> MYGTGTGPQTGAVTPRSSASLRPLTLSHGSLETSFLIPTGLHFHASRLKDEFIASLPPPTDELAQDDEPSSVPELVARYMGYIANQVAEGEDDAQGSYEEVLKLILNEFERAFLQGNDVHALVATLPGIDAKKLEVIRSYFAARAATNRAMRAHQSALLRAAEEGEARIYSIFGGQGNIEEYFEELRELYKTYPSFVGHLIVSSAELLQILASHPSAEKLYSKGLDIMHWLHNPDATPDTDYLISAPVSFPLIGLVQLAHYQVTCKVQGLHPGILRDRISGTTGHSQGIVLAAVTAAADSWESFEDLAKSALTILFWIGARSQQTFPRTSMSPSLLQEAIDNGEGTPTPMLSIRDLPQAEVQKHIDQTNQYLPEDQHISISLINSPRNLVVSGPPRSLCGLNAQLRKVKAPTGLDQARIPYSERKIRFVNRFLPITAPFHSKYLAGAAELIAEDLKDISIEVERLGIPVYDTNTGEDIRQTVTGNVVPALIRMITNDPVHWEKATVFPEATHILDFGPGGISGLGVLTSRNKDGTGVRVILAGTVNGTVAEVGYKSELFDRDEEHAVKYAVDWVKEYGPRLIKTSSGRIYVDTKMSRLLGLPPLMVAGMTPTTVPWDFVAATMNAGYQIELAGGGYFNAKMMTEAISKIERAIPPGRGITVNLIYVNPHAMAWQIPLLGRLRAEGVPIEGLTIGAGVPSIEVANEYIQTLGLKHISFKPGSVDAIQAVINIAKANPTFPVILQWTGGRGGGHHSYEDFHAPILAMYSRIRRQENIILVAGSGFGGAEDTYPYLTGAWSTKYGYPPMPFDGCLFGSRMMVAKEAHTSPEAKQAIVDAPGLDDSEWEKTYKGPAGGVITVRSEMGEPIHKLATRGVLFWAEMDQKIFSLPKEKRVAELKKNRDYIIRKLNADFQKVWFGKNKKGEVVDLEDMTYGEVVRRMVELLYVKDEKRWIDHSFAKLTADFIHRVEERFTTAASQPSLIQSYSDLDEPYSAVERVLAHYPEAETQLISAQDVQHFLLLCKRRGQKPVTFVPALDEDFEFYFKKDSLWQSEDLAAVIDRDVGRTCILQGPMAAKHSTKVDEPIKEILDGIHNGHIAALKRDLYDNDESKIPTIEYFGGKLKDPEVQLDFEGVTISYDVHKNTYRVSNNPSVPLPPLDAWLSALAGPNRTWRYALLQSEVIVQGHKYQTNPMKKIFAPARGLFVEIQYPNDPAKTVITVKEQPRPNRYIDVIEAKLVGDKEIVVNLIKDTNALGEPVALPLRFTYRPEAGYAPIHEIMEGRNDRIKEFYWRCWFGQDPLDLDAPVTSKFDGGEAVITSEAINEFVHAVGNTGEAFVDRPGKTMYAPMDFAIVVGWKAITKPIFPRTIDGDLLKLVHLSNQFRMFPGAEPLKKGDKVYTTAQVNAVINQESGKMVEVCGTITRDGKPVMEVISQFLYRGVYTDYENTFQRKVETPMQVHLATTKDIAILRSKQWFVLDDVATPEEFLLGKTLTFRLHTLVHFKNRNVYSHVETRGQVLVELPTKEIIQVATVEYVAGESHGNPVIDYLQRNGQSIEQPVNFENPIPLGGKAPLQLRAPASNETYARVSGDYNPIHVSRVFAAYANLPGTITHGMYSSAAVRSLVETWAAENKIGRVRSFHASLTGMVLPNDDINVKLQHVGMVGGRKIIKVEATNKETEEKVLLGEAEIEQPVTAYVFTGQGSQEQGMGMDLYANSPVAREVWDRADKYLRDTYGFAITDIVRNNPKELTIHFGGPLGKKIRANYMAMTFETVAADGSIKSERIFKDIDENTTSYTFRSPNGLLSATQFTQPALTLMEKASFEDMKAKGLVPRDSTFAGHSLGEYSALAALADVMPIESLVSVVFYRGLTMQV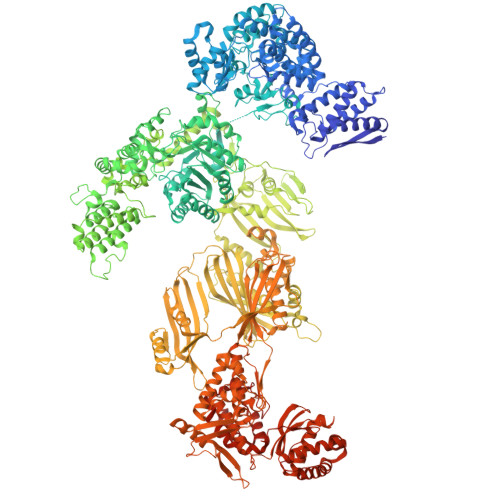AVERDATGRSNYGMCAVNPSRISKTFNEEALRFVVGAVAETTGWLLEIVNYNIANMQYVCAGDLRALDTLTSVTNFIKAMKIDIEQMRREYSPDKVKEELVEIIKKCAAETEAKPKPLELQRGFATIPLRGIDVPFHSTFLRSGVKPFRNFLLKKINKTSIDPAKLIGKYIPNVTAKPFALTKEYFEDVYRLTNSPRIAHVLANWEKYQDDNSTLSASVANTSSETNGVNGVNGAVDVNGQNGVNGVNGH Syncrip is a conserved RNA-binding protein important in neuronal and muscular development in Drosophila and mammals. In the fly embryo, Syncrip is important for the morphology and growth of the neuromuscular junction and regulates cytoplasmic vesicle-based messenger RNA (mRNA) transport. Importantly, we showed that Syncrip recognises an hEXO (GGCU/A) sequence in a set of miRNA targets and mediates their exosomal enrichment. We identify a cryptic RNA-binding unit that recognises RNA with high-sequence specificity and show that this non-canonical RNA-binding domain is responsible for hEXO recognition in Syncrip-mediated exosomal miRNA partitioning.

In order to investigate the non-canonical N-terminal RNA-binding region of Syncrip and to provide a structural framework for our studies, we set out to determine the structure of the N-terminal region of the conserved N-terminal ‘acidic’ and RRM1 domains (NeR1 construct) in Human and Drosophila Syncrip proteins. The Drosophila protein crystallised in space group P21 with two copies in the asymmetric unit. The 2.2 Å resolution X-ray structure was solved by single-wavelength anomalous diffraction (SAD) using a seleno-methionine derivatised protein. Finally, we observed that two high-confidence and five candidate RNA-bound peptides mapped to the amino (N)-terminal region of Syncrip, overlapping with the ‘acidic’ domain that has previously been described as a putative protein-interaction unit. The presence of multiple high-confidence RNA-bound peptides in this region indicates it likely plays a role in the interaction with target RNAs in the cell. Analysis of the Syncrip sequence with this algorithm revealed high-probability RNA-binding activities not only in the RRMs, but also in the ‘acidic’ N-terminal domain. This indicates that the N-terminal ‘acidic’ domain, although specific to Syncrip protein, contains patterns of short sequences often associated with RNA-binding sites in other proteins. We also show that the domain is functionally and physically coupled by a structural element to a second RNA-binding region comprising the RRM domains, and that the coordinated interaction of multiple Syncrip RNA-binding domains is the basis of efficient recognition of the full-length miRNA.

>GERTEDYPKLLEYGLDKKVAGKLDEIYKTGKLAHAELDERALDALKEFPVDGALNVLGQFLESNLEHVSNKSAYLCGVMKTYRQKSRASQQGVAAPATVKGPDEDKIKKILERTGYTLDVTTGQRKYGGPPPHWEGNVPGNGCEVFCGKIPKDMYEDELIPLFENCGIIWDLRLMMDPMTGTNRGYAFVTFTNREAAVNAVRQLDNHEIKPGKCLKINISVP[2x]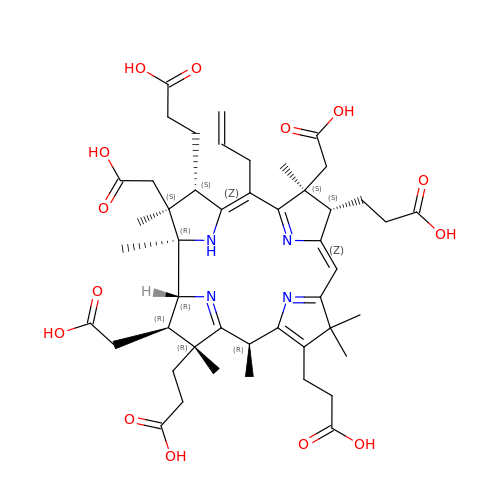3-[(1~{R},2~{S},3~{S},4~{Z},7~{S},8~{S},9~{Z},15~{R},17~{R},18~{R},19~{R})-2,7,18-tris(2-hydroxy-2-oxoethyl)-3,13,17-tris(3-hydroxy-3-oxopropyl)-1,2,7,12,12,15,17-heptamethyl-5-prop-2-enyl-3,8,15,18,19,21-hexahydrocorrin-8-yl]propanoic acid | C47 H62 N4 O14 | VXYZYIAZOLQLTR-JBBZEPTESA-N(1S)-1,5-anhydro-1-(3-{4-[hydroxy(oxo)azaniumyl]phenyl}-1H-1,2,4-triazol-5-yl)-D-glucitol 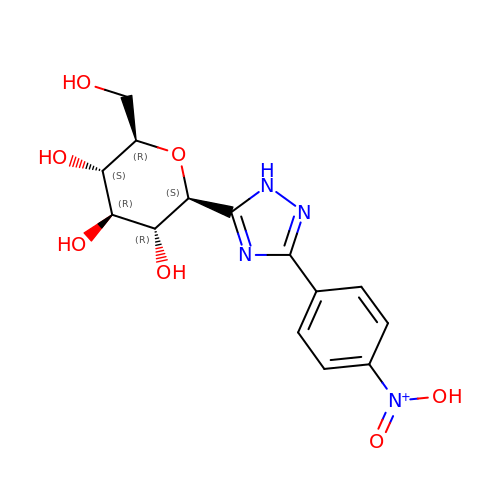| C14 H17 N4 O7 | UCUAXDZFQJPZOC-RMPHRYRLSA-N>MSQPITRENFDEWMIPVYAPAPFIPVRGEGSRLWDQQGKEYIDFAGGIAVNALGHAHPELREALNEQASKFWHTGNGYTNEPVLRLAKKLIDATFADRVFFCNSGAEANEAALKLARKFAHDRYGSHKSGIVAFKNAFHGRTLFTVSAGGQPAYSQDFAPLPADIRHAAYNDINSASALIDDSTCAVIVEPIQGEGGVVPASNAFLQGLRELCNRHNALLIFDEVQTGVGRTGELYAYMHYGVTPDLLTTAKALGGGFPVGALLATEECARVMTVGTHGTTYGGNPLASAVAGKVLELINTPEMLNGVKQRHDWFVERLNTINHRYGLFSEVRGLGLLIGCVLNADYAGQAKQISQEAAKAGVMVLIAGGNV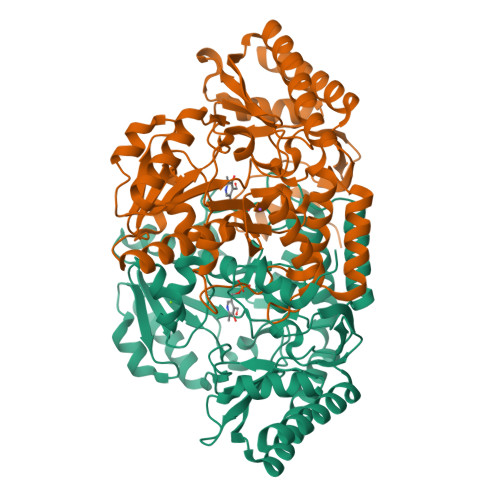VRFAPALNVSEEEVTTGLDRFAAACEHFVSRGSS[4x]> GSHMDNQCTVQVRLELGHRAQLRKKPTTEGFTHDWMVFVRGPEQCDIQHFVEKVVFWLHDSFPKPRRVCKEPPYKVEESGYAGFIMPIEVHFKNKEEPRKVCFTYDLFLNLEGNPPVNPLNHLRCEKLT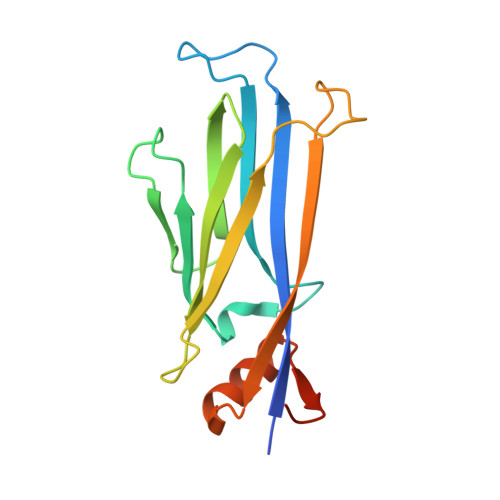FNNPTTEFRYKLLRAGGVMVMPEGAHHHHHH> MTTVESNTTAAIPDEIARQIVLPEGHKDNVPLFEAYRWLRENQPLGQARVEGYDPLWLITKYADLMEVERQ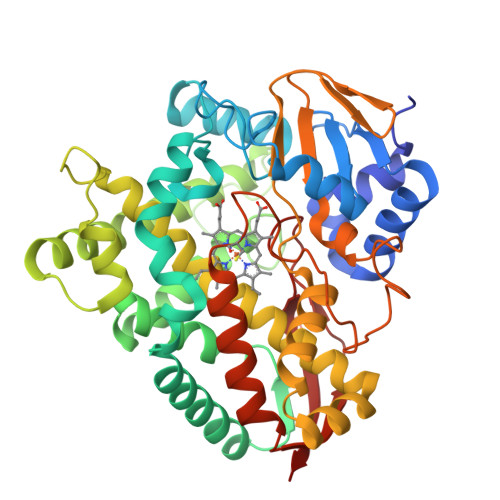PQIFAAGGGEDKGSNNPILANQAGDEFTRQLLGGNLRILDALPYLDQPEHSVVKDVAFDWFRPANLKKWEDRIRETARASIDRLLAGGPDLDAVQEFAVFFPLRVIMSLFGVPEEDEPRMMALTQDFFGVADPDAQRDDIEALSPDAAAQQWAATIADFYAYFDVLVESRRAEPRDDLATLIAVAKDENGEYFPKTFAYGWFVAIATAGHDTTASTLAGCLQSLAAHPEVLDRVKGDPDLIPDLVNESLRIVSPVKHFTRVALQDYEMRGQKIKAGDRLMLLFQSGNRDAEVFDRPDDFDIDRRPNKHIAFGYGPHMCIGQHLAKLELKVMLQELLPHLERVEVSGEPKLIQTNFVGGLRKLPVHLTFS>[2x]HMERPESELIRQSWRVVSRSPLEHGTVLFARLFALEPSLLPLFGSSPEFLDHIRKVMLVIDAAVTNVEDLSSLEEYLTSLGRKHRAVGVRLSSFSTVGESLLYMLE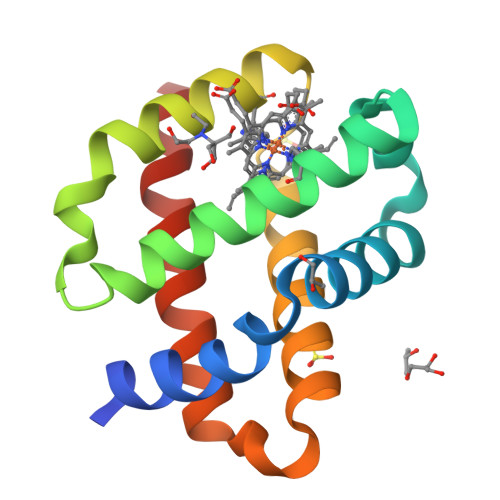KSLGPDFTPATRTAWSRLYGAVVQAMSRGWDGE> SRSKRDNNFYSVEIGDSTFTVLKRYQNLKPIGSGAQGIVCAAYDAILERNVAIKKLSRPFQNQTHAKRAYRELVLMKCVNHKNIIGLLNVFTPQKSLEEFQDVYIVMELMDANLCQVIQMELDHERMSYLLYQMLCGIKHLHSAGIIHRDLKPSNIVVKSDCTLKILDFGLARTAGTSFMMT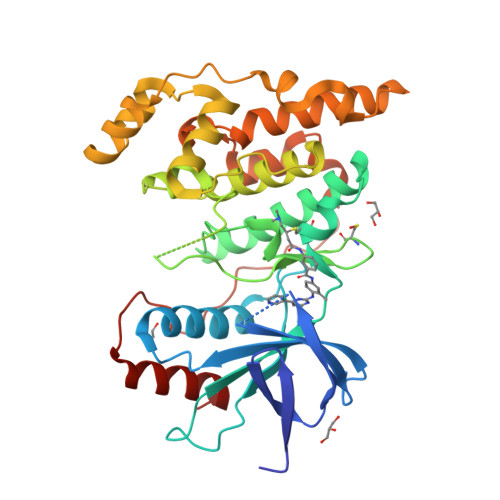PYVVTRYYRAPEVILGMGYKENVDIWSVGCIMGEMIKGGVLFPGTDHIDQWNKVIEQLGTPCPEFMKKLQPTVRTYVENRPKYAGYSFEKLFPDVLFPADSEHNKLKASQARDLLSKMLVIDASKRISVDEALQHPYINVWYDPSEAEAPPPKIPDKQLDEREHTIEEWKELIYKEVMDLE Multidrug resistance-associated protein 2 (MRP2/ABCC2) is a polyspecific efflux transporter of organic anions expressed in hepatocyte canalicular membranes. MRP2 (multidrug resistance-associated protein, 2) is a primary active transporter of the ATP-binding cassette (ABC) class. We have built an atomic model for rMrp2 that consists of a small N-terminal transmembrane domain (TMD0) that is linked to two transmembrane domains (TMD), TMD1 and TMD2, by the lasso linker (L0). Each TMD consists of 6 TM helices, enclosing the pocket for substrates and drugs binding, and they are linked to two nucleotide binding domains (NBDs), NBD1 and NBD2, where ATP binding and hydrolysis provides the free energy required for the transport cycle completion.

In the absence of nucleotides, rMrp2 adopts an inward-facing conformation with the TMDs open to the cytosol where substrates and drugs can access it. An unusual feature of the rMrp2 cryo-EM maps was the presence of helical-like density within the TMD1 and TMD2 interface that corresponds to the regulatory domain (R-domain); MRP2 and other members of the ABCC family contain an R-domain that regulates their transport activity upon phosphorylation by specific kinases (CKII, PKC, PKA and PLK kinases). The R-domain is predicted to be partly helical from the AlphaFold2 model and it links NBD1 to the elbow helix (short helix at the amine-terminal of TM12 and it sits perpendicular to the TMD2), but in the predicted model it was placed at the interface of the NBDs and outside the TMD whereas in our structure it sits deep inside the TMD. Although, continuous density from NBD1 to the helical density can be observed, only the helical part, residues Ala895-Lys924, was modelled as the rest of the density is weak and without defined side chains; in addition, there is no density that links the C-terminus of the R-domain to the elbow helix. The R-domain is buried within the TMDs at the interface of TMs 8, 9, 11 and 17 and it is stabilised by several hydrogen bonds and Van der Waals interactions. As the R-domain of rMrp2 is deep inside the TMD1/2 interface, it points to an inactive conformation that would prevent bilirubin glucuronide or drug binding and the formation of an NBD:NBD interface. Since the R-domain in our cryo-EM structure is partially phosphorylated, Thr869, Ser874 and Thr886, it suggests that phosphorylation of these residues does not relieve autoinhibition (full dephosphorylation of rMrp2 did not alter the ATP hydrolysis kinetics either), but their role might be to stabilise the R-domain. Although the R-domain is observed deep inside the TMD of the rMRP2 structure, our functional data show that rMrp2 retains its ATPase activity adding further support for the concept of the R-domain equilibrium.

> MDKFCNSTFWDLSLLESPEADLPLCFEQTVLVWIPLGFLWLLAPWQLYSVYRSRTKRSSITKFYLAKQVFVVFLLILAAIDLSLALTEDTGQATVPPVRYTNPILYLCTWLLVLAVQHSRQWCVRKNSWFLSLFWILSVLCGVFQFQTLIRALLKDSKSNMAYSYLFFVSYGFQIVLLILTAFSGPSDSTQTPSVTASFLSSITFSWYDRTVLKGYKHPLTLEDVWDIDEGFKTRSVTSKFEAAMTKDLQKARQAFQRRLQKSQRKPEATLHGLNKKQSQSQDVLVLEEAKKKSEKTTKDYPKSWLIKSLFKTFHVVILKSFILKLIHDLLVFLNPQLLKLLIGFVKSSNSYVWFGYICAILMFAVTLIQSFCLQSYFQHCFVLGMCVRTTVMSSIYKKALTLSNLARKQYTIGETVNLMSVDSQKLMDATNYMQLVWSSVIQITLSIFFLWRELGPSILAGVGVMVLLIPVNGVLATKIRNIQVQNMKNKDKRLKIMNEILSGIKILKYFAWEPSFQEQVQGIRKKELKNLLRFGQLQSLLIFILQITPILVSVVTFSVYVLVDSANVLNAEKAFTSITLFNILRFPLSMLPMVTSSILQASVSVDRLERYLGGDDLDTSAIRRVSNFDKAVKFSEASFTWDPDLEATIQDVNLDIKPGQLVAVVGTVGSGKSSLVSAMLGEMENVHGHITIQGSTAYVPQQSWIQNGTIKDNILFGSEYNEKKYQQVLKACALLPDLEILPGGDMAEIGEKGINLSGGQKQRVSLARAAYQDADIYILDDPLSAVDAHVGKHIFNKVVGPNGLLAGKTRIFVTHGIHFLPQVDEIVVLGKGTILEKGSYRDLLDKKGVFARNWKTFMKHSGPEGEATVNNDSEAEDDDDGLIPTMEEIPEDAASLAMRRENSLRRTLSRSSRSSSRRGKSLKNSLKIKNVNVLKEKEKEVEGQKLIKKEFVETGKVKFSIYLKYLQAVGWWSILFIILFYGLNNVAFIGSNLWLSAWTSDSDNLNGTNNSSSHRDMRIGVFGALGLAQGICLLISTLWSIYACRNASKALHGQLLTNILRAPMRFFDTTPTGRIVNRFSGDISTVDDLLPQTLRSWMMCFFGIAGTLVMICMATPVFAIIIIPLSILYISVQVFYVATSRQLRRLDSVTKSPIYSHFSETVTGLPIIRAFEHQQRFLAWNEKQIDINQKCVFSWITSNRWLAIRLELVGNLVVFCSALLLVIYRKTLTGDVVGFVLSNALNITQTLNWLVRMTSEAETNIVAVERISEYINVENEAPWVTDKRPPADWPRHGEIQFNNYQVRYRPELDLVLKGITCNIKSGEKVGVVGRTGAGKSSLTNCLFRILESAGGQIIIDGIDVASIGLHDLRERLTIIPQDPILFSGSLRMNLDPFNKYSDEEVWRALELAHLRSFVSGLQLGLLSEVTEGGDNLSIGQRQLLCLGRAVLRKSKILVLDEATAAVDLETDSLIQTTIRKEFSQCTVITIAHRLHTIMDSDKIMVLDNGKIVEYGSPEELLSNRGSFYLMAKEAGIENVNHTEL>MEEPEEPADSGQSLVPVYIYSPEYVSMCDSLAKIPKRASMVHSLIEAYALHKQMRIVKPKVASMEEMATFHTDAYLQHLQKVSQEGDDDHPDSIEYGLGYDCPATEGIFDYAAAIGGATITAAQCLIDGMCKVAINWSGGWHHAKKDEASGFCYLNDAVLGILRLRRKFERILYVDLDLHHGDGVEDAFSFTSKVMTVSLHKFSPGFFPGTGDVSDVGLGKGRYYSVNVPIQDGIQDEKYYQICESVLKEVYQAFNPKAVVLQLGADTIAGDPMCSFNMTPVGIGKCLKYILQWQLATLILGAGGY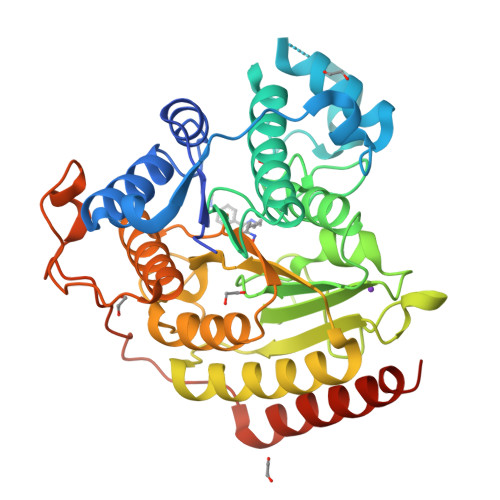NLANTARCWTYLTGVILGKTLSSEIPDHEFFTAYGPDYVLEITPSCRPDRNEPHRIQQILNYIKGNLKHVVIEGRGSHHHHHH[4x]> MEVYRRITERVRGALWAHHGRLMSERQFHRILAFVYNNKYEYQIRFDRMEVVGREWGGRVEVVTTPAGFLKRVRVNPCVEDLTLYQQQQLILSAYANACADGRKLMEQAEMNIYKQFLKDLKPIVMGIRDNPEFYTVSENSIETIGGVLQTG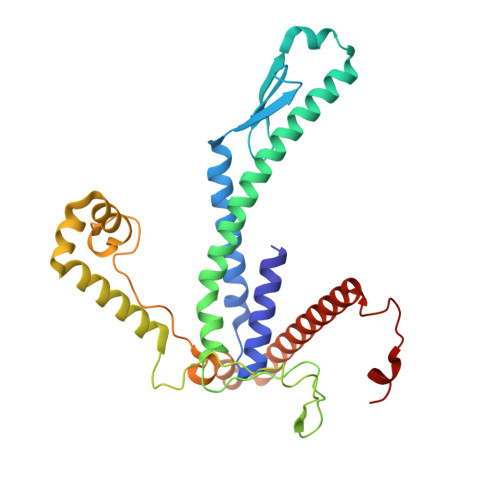DSNNLCHTHRTIPAAKARQPADEVRARQEWEQKWINSPRGQSWALTLRGKTYFALHGPQYRPRGAPGAKKETLPLDIPAPYTAMDEKRLLKKNWMAYLDNKHVAEVMWTRVKIADREKRQRLLQETGRAWHRPINEEAINRW>EFMAPKVLFIHNEHMCTEAMLGDAFSECGFDIETFEVVPPERVETPAGDVAFPDPTAYDVIVPLGARWPVYEQSLVGTWVTAEMDMMRKAADAGVGILGVCFGGQLLAQTFGGSVARAETAEVGWFELDTDDAGLIAPGPWFQWHFDRWTVPPGATEIARTSRSSQAFVLGRALALQFHPEVDVDLLEGWLADDREGISGKLGYNHDDLRL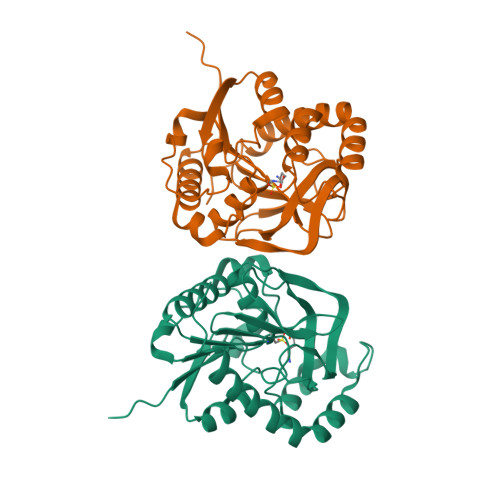RTKELVDDAAVRVRELVRAFLDKVVRADPAS[2x]>[4x]HMAVKKIAIFGATGQTGLTTLAQAVQAGYEVTVLVRDSSRLPSEGPRPAHVVVGDVLQAADVDKTVAGQDAVIVLLGTRNDLSPTTVMSEGARNIVA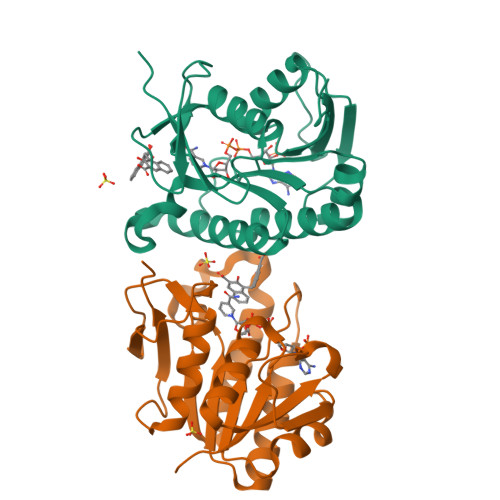AMKAHGVDKVVACTSAFLLWDPTKVPPRLQAVTDDHIRMHKVLRESGLKYVAVMPPHIGDQPLTGAYTVTLDGRGPSRVISKHDLGHFMLRCLTTDEYDGHSTYPSHQYQ> DDHSELLVNTKSGKVMGTRVPVLSSHISAFLGIPFAEPPVGNMRFRRPEPKKPWSGVWNASTYPNNCQQYVDEQFPGFSGSEMWNPNREMSEDCLYLNIWVPSPRPKSTTVMVWIYGGGFYSGSSTLDVYNGKYLAYTEEVVLVSLSYRVGAFGFLALHGSQEAPGNVGLLDQRMALQWVHDNIQFFGGDPKTVTIFGESAGGASVGMHILSPGSRDLFRRAILQSGSPNCPWASVSVAEGRRRAVELGRNLNCNLNSDEELIHCLREKKPQELIDVEWNVLPFDSIFRFSFVPVIDGEFFPTSLESMLNSGNFKKTQILLGVNKDEGSFFLLYGAPGFSKDSESKISREDFMSGVKLSVPHANDLGLDAVTLQYTDWMDDNNGIKNRDGLDDIVGDHNVICPLMHFVNKYTKFGNGTYLYFFNHRASNLVWPEWMGVIHGYEIEFVFGLPLVKELNYTAEEEALSRRIMHYWATFAKTGNPNEPHSQESKWPLFTTKEQKFIDLNTEPMKVHQRLRVQMCVFWNQFLPKLLNATAC

Stabilization of Torpedo californica acetylcholinesterase by the divalent cations Ca+2, Mg+2, and Mn+2 was investigated. All three substantially protect the enzyme from thermal inactivation. Differential scanning calorimetry showed a single irreversible thermal transition. All three cations raise both the temperature of the transition and the activation energy, with the transition becoming more cooperative.

The crystal structures of the Ca+2 and Mg+2 complexes with Torpedo acetylcholinesterase were solved. A principal binding site was identified. In both cases, it consists of four aspartates (a 4D motif), within which the divalent ion is embedded, together with several water molecules. It makes direct contact with two of the aspartates, and indirect contact, via waters, with the other two. The ASSAM server retrieved 200 other proteins that display the 4D motif, in many of which it is occupied by a divalent cation. It is a very versatile motif, since, even though tightly conserved in terms of RMSD values, it can contain from one to as many as three divalent metal ions, together with a variable number of waters.>MGHHHHHHAENLYFQGADPMSKLSDSKSVFSKLSNKQIETIIQRYASPCFIIDENALLERARLFQQAILNQYQNSIAAYSVKTQSLNTIIQKFYEVGFIPEVVSSDEFEQIQKLQLCDKSIIFNGPYKNDASLIKALQLNAMINCDHFDEILRIAKIAKKLNITAKIGLRIADNKTPQNWSRFGFALTDQQNNSDIFTTIDKIQQIANIQLAGLHCHIGTNIRDISRFTAMAKNIAELAETILTKYKLTLEWIDLGGGLAGISPTLSDKRLQPYNPFDLELYAATIIAPLKEYLNKTNDKTKLIFELGRSLVDYSVALLTTIVGTREQNEDFQSLITDAGIHTIPTISTYRHPIYHLKTDSYHKKTLLLGPSCMQHDFLHDDIFLPKLEYGDKLLIDGVGAYNISRNNEFIHLKPSVI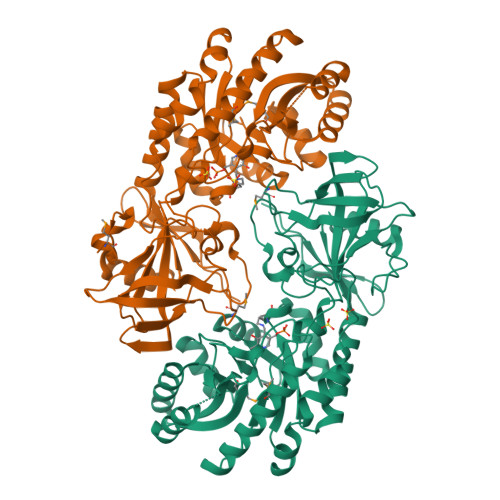LIDKNQQYQVLRVRQTHQ[4x]>MCNTNMSVPTDGA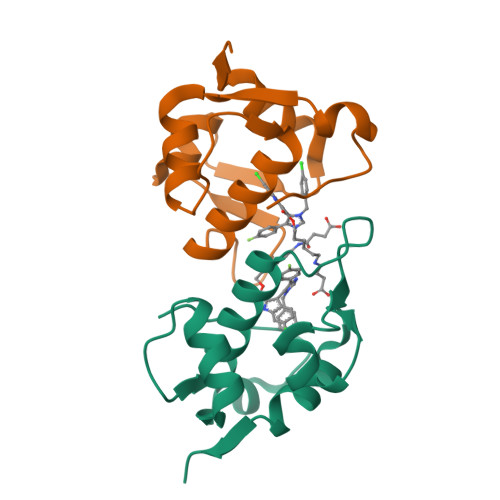VTTSQIPASEQETLVRPKPLLLKLLKSVGAQKDTYTMKEVLFYLGQYIMTKRLYDEKQQHIVYCSNDLLGDLFGVPSFSVKEHRKIYTMIYRNLVVVNQQESSDSGTSVSEN[4x]(4S,5R)-4-hydroxy-5-methyl-5-[(1-phenyl-1H-1,2,3-triazol-4-yl)methyl]pyrrolidin-2-one 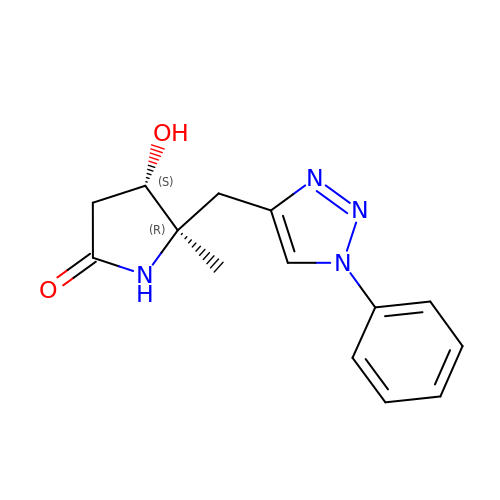| C14 H16 N4 O2 | UILOQPSPJQYNHO-GXTWGEPZSA-N>DTMKVINDPIHGHIELHPLLVRIIDTPQFQRLRYIKQLGGGYYVFPGASHNRFEHSLGVGYLAGCLVHALGEKQPELQISERDVLCVQIAGLCRNLGHGPFSHMFDGRFIPLARPEVKWTHEQGSVMMFEHLINSNGIKPVMEQYGLIPEEDICFIKEQIVGPLESPVEDSLWPYKGRPENKSFLYEIVSNKRNGIDVDKWDYFARDCHHLGIQNNFDYKRFIKFARVCEVDNELRIC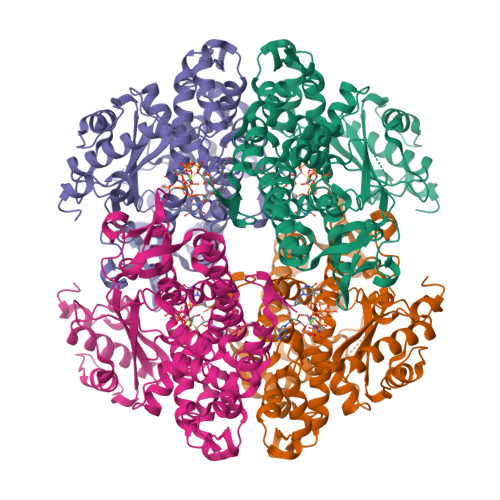ARDKEVGNLYDMFHTRNSLHRRAYQHKVGNIIDTMITDAFLKADDYIEITGAGGKKYRISTAIDDMEAYTKLTDNIFLEILYSTDPKLKDAREILKQIEYRNLFKYVGETQPTGQIKIKREDYESLPKEVASAKPKVLLDVKLKAEDFIVDVINMDYGMQEKNPIDHVSFYCKTAPNRAIRITKNQVSQLLPEKFAEQLIRVYCKKVDRKSLYAARQYFVQWCADRNFTKPQDGDVIAPLITPQKKEWNDSTSVQNPTRLREASKSRVQLFKDDPM[4x]>IVGGSDAKEGAWPWVVGLYYDDRLLCGASLVSSDWLVSAAHCVYGRNLEPSKWTAILGLHMKSNLTSPQTVPRLIDEIVINPHYNRRRKDNDIAMMHLEFKVNYTDYIQPISLPEENQVFPPGRNCSIAGWGTVVYQGTTADILQEADVPLLSNERCQQQMPEYNI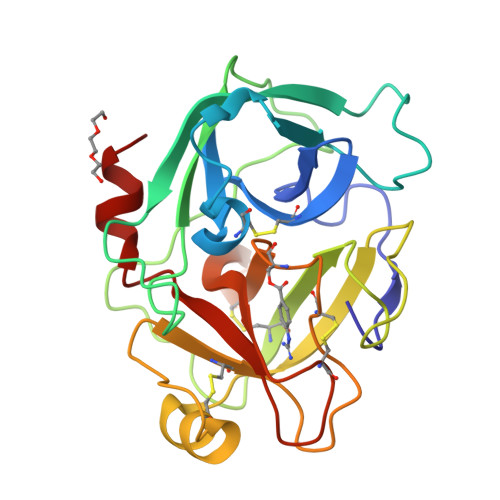TENMICAGYEEGGIDSCQGDSGGPLMCQENNRWFLAGVTSFGYECALPNRPGVYARVSRFTEWIQSFLH[4x]> MLQQVFGKSKGGEVTNSHLTPKVLNKAQEAEKLASQIQAQRFSNRLVAFSSQYPRAKLFFAGIGIGTLLYGANQSSKARENKVATETRKERMAKPTIQLTGADSQNPPFTEKNINDWLYKTVSITGRPIHGKGMMIPAKSYGLHGFEYLVPFVTKEN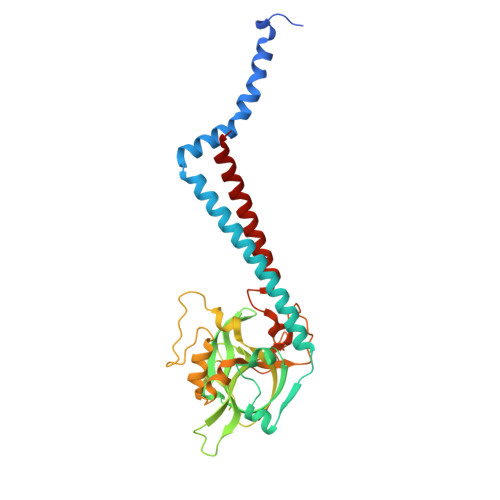EDGSVQEGLILNLGFIPREYAPIWARARVENVEEQTFTCVVTDGKHLSEQGGLFASNKPCENQWEYADLDQLAKHTGFVNQEQVRSCILEHVNTETPNDERDCRHIDICSDYKEDYPYKFTRSGVLQQPGQMYWDLNKSASYYSLLGLGCSVFSALLFLAK>MAAKLWTFLLGFGLSWVWPASAHRKLLVLLLDGFRSDYISEDALASLPGFREIVNRGVKVDYLTPDFPSLSYPNYYTLMTGRHCEVHQMIGNYMWDPRTNKSFDIGVNRDSLMPLWWNGSEPLWITLMKARRKVYMYYWPGCEVEILGVRPTYCLEYKTVPTDINFANAVSDALDSLKSGRADLAAIYHERIDVEGHHYGPSSPQRKDALRAVDTVLKYMIQWIQDRGLQQDLNVILFSDHGMTDIFWMDKVIELSNYISLDDLQQVKDRGPVVSLW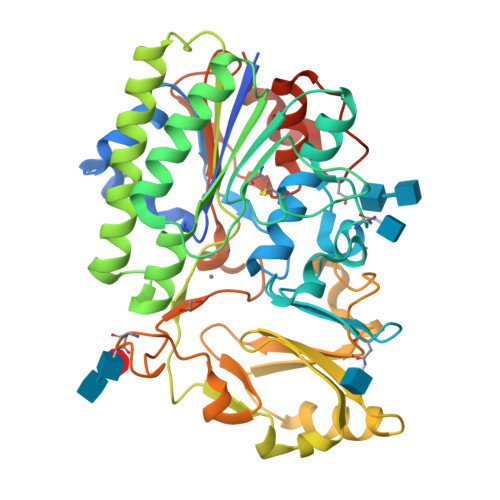PVPGKHSEIYHKLRTVEHMTVYEKESIPNRFYYKKGKFVSPLTLVADEGWFIAESREMLPFWMNSTGKREGWQRGWHGYDNELMDMRGIFLAIGPDFKSNFRAAPIRSVDVYNIMAHVAGITPLPNNGSWSRVVSMLKGQTSSASRENLYFQ[4x]>NVHSNYTFIIAGGGISGLTLADRLTEDPRVTVLVIEAGPLDRGEDGILVPGAFSPWLYFWPGLVSTPQAGLNNRTVDVITAQVVGGGSTINAMVYLRGDKDDYDSWGALGNPGWSWNSMLPYFIKSETFTPPSPELAAAGNITWDGSIRGRSGPVNYSYPNYFFPGSENWWNAANEVGLPPVKDPMAGSKQGVFWIPSAIDARTMTRSHARRNHYDRVSSRPNYHILPSHLVSKILFRGKQAIGVSYIPTSGGNTTTNVYASKEITLAAGGLGTPKILQLSGIGPRKLLNELGIPVISDLPGVGQNLQDQPTLTIPYTFTNNVFPNTDSLTTNATYNAEQRALYDSSKQGAYTIVNSLSTNIGVMSLQRAAPKSYRQIIAAARARSASLSLPPGTDPAVIRGYQAQRNAILKQFENPNV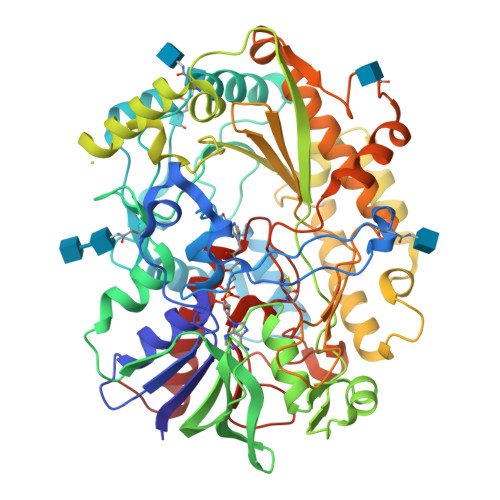GVGTVHWGTGSSALVYHLKPLSRGTVNIRSTNPLDAPEIDYRTGTDPIDAQVYTSLFRKNREIFNAPSMRVLGPSEAAPFGANLTTDEEIYAVMRELINPSNAHQCCTAAMMPKDMGGVVSSEQKVYGVQGLRVADISFWPFQLSGSPMATAYAGAERLADVIKKEHRLAGAPKSL[2x]> G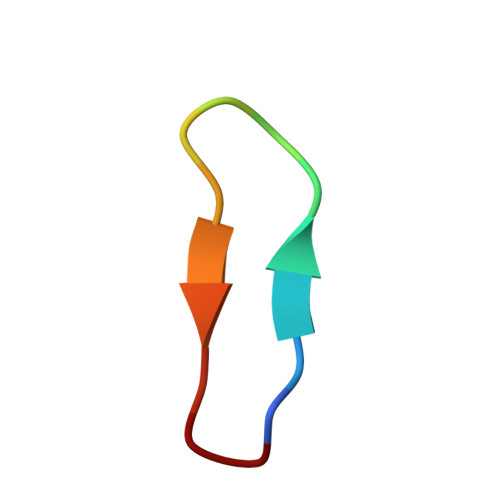RAYKSKPPIAFPD>GTKRPFRQNLNPLVLLLDAALTGELEVVQQAVKEMNDPSQPNEEGITALHNAICGANYSIVDFLITAGANVNSPDSHGWTPLHCAASCNDTVICMALVQHGAAIFATTLSDGATAFEKCDPYREGYADCATYLADVEQSMGLMNSGAVYALWDYSAEFGDELSFREGESVTVLRRDGPEETDWWWAALHGQEGYVPRNYFGLFPRVKPQR[4x]

The ASPP family of proteins is involved in modulating the transcriptional activity of the p53 protein family members, including p63. Despite their antagonizing functions, the ASPP family members share a highly homologous C‐terminal domain (CTD) which mediates the direct interaction with p53 and consists of four ankyrin repeats (ARs) conjoined with an SH3 domain. Here we characterize the interaction of iASPP with p63 and show that it binds to the linker region between the DNA binding domain and the oligomerization domain. We further demonstrate that this binding site is removed in a splice variant of p63 where a stretch of five amino acids is replaced with a single alanine residue. This stretch contains a degenerate class II SH3 domain binding motif that is responsible for interaction with iASPP, as well as two positively charged amino acids.

We wanted to investigate the structural details of the interaction and solved the crystal structure of the iASPP CTD in complex with the p63 linker peptide. Since the KD for the interaction is with ~90 µM relatively weak, we fused the p63 peptide (amino acids 332‐342) directly to the iASPP CTD (amino acids 625‐828). In the crystal structure, the p63 peptide of one fusion protein bound to the SH3 domain of a neighboring protein of the asymmetric unit. The p63 peptides of all four chains present within the asymmetric unit of the crystal lattice adopted an almost identical conformation with differences only in the orientation of T335, Q341 and F339. No electron density was observed for G332 and D333 at all, whereas G334 was only resolved in one chain. In detail, the p63 peptide adopted the conformation of a class II SH3 domain binding motif (PxφPx + ) despite the lack of one proline. P338 occupied the second xP pocket, whereas R340 contacted D775 and E776 of the RT loop and E795 of the n‐src loop which make up the acidic region of the SH3 domain. p63 R337, at the position of the aliphatic residue in the canonical class II motif, interacted with the RT loop as well by reaching towards E776 of the acidic region. The aliphatic moiety of the K336 side chain partially occupied the first xP pocket. The proximity of the W767 side chain could also allow for a cation‐π interaction via the ε‐amino group of K336. The ankyrin repeats (ANK1 to ANK4, dark grey) do not contribute to the interaction.>[2x]UUGGGCCA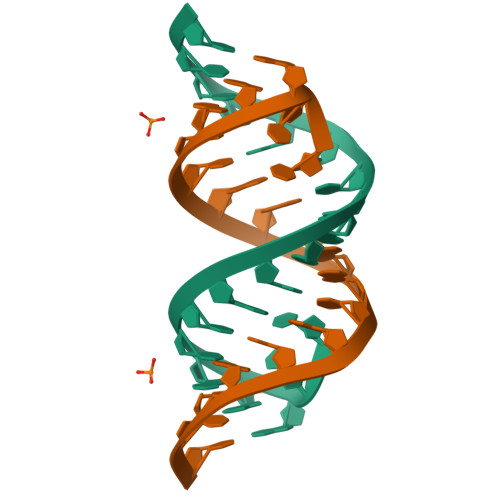GCAGCAGGUCC> SNANFDTNMFKLENYVKEKYSLESLEIIPNEFDDTPTILSERISQVAAGVLRNLIDDNMKIGFSWGKSLSNLVDLIHSKSVRNVHFYPLAGGPSHIHAKYHVNTLIYEMSRKFHGECTFMNATIVQENKLLADGILQSRYFENLKNSWKDLDIAVVGIGDFSNKGKHQWLDMLTEDDFKELTKVKTVGEICCRFFDSKGKEVYENLQER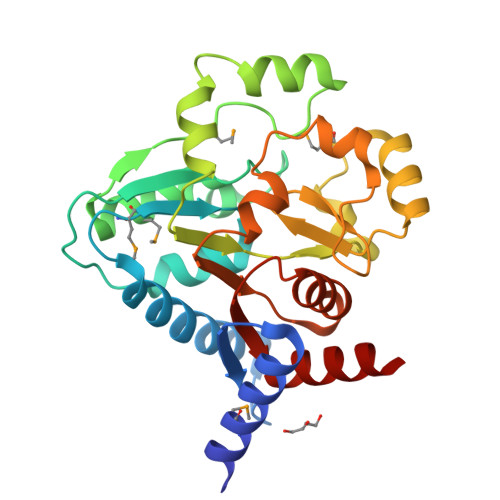TIAISLEDLKNIPQSLAVAYGDTKVSSILSVLRANLVNHLITDKNTILKVLEEDGDL N-{(3R)-1-[(4-chlorophenyl)methyl]pyrrolidin-3-yl}-2-(3-methoxyphenyl)-N-methylquinoline-4-carboxamide | 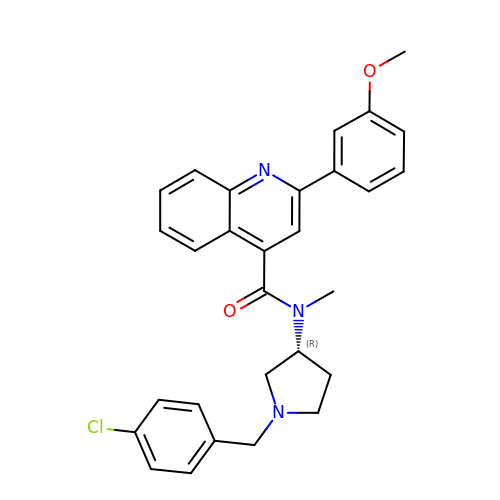C29 H28 Cl N3 O2 | UPCGOPZWVBKZPL-HSZRJFAPSA-N> MLKFML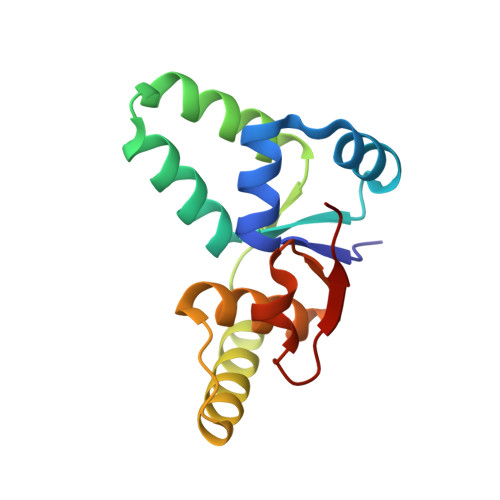DTNTCIFTIKNKPEHIRERFNLNTSRMCISSITLMELIYGAEKSLAPERNLAVVEGFISRLEVLDYDTQAAIHTGQIRAELARKGTPVGPYDQMIAGHAGSRGLVVVTNNLREFERIPGIRIEDWC>MLIRRLKDARLRAGISQEKLGVLAGIDEASASARMNQYEKGKHAPDFEMANRLAKVLKIPVSYLYTPEDDLAQIIL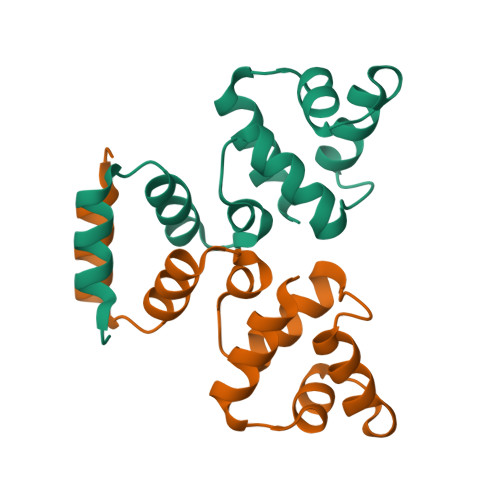TWNELNEQERKRINFYIRKKAK[2x]> GPPPRFQRDFVDLRTDCPSTHPPIRVMQWNILAQALGEGKDNFVQCPVEALKWEERKCLILEEILAYQPDILCLQEVDHYFDTFQPLLSRLGYQGTFFPKPWSPCLDVEHNNGPDGCALFFLQNRFKLVNSANIRLTAMTLKTNQVAIAQTLECKESGRQFCIAVTHLKARTGWERFRSAQGCDLLQNLQNITQGAKIPLIVCGDFNAEPTEEVYKHFASSSLNLNSAYKLLSADGQSEPPYTTWKIRTSGECRHTLDYIWYSKHALNVRSALDLLTEEQIGPNRLPSFNYPSDHLSLVCDFSFTEESDGLS

A screen for circadian genes using Xenopus laevis retinas identified the ~50 kDa protein Nocturnin (NOCT), which exhibited a rhythmic expression that peaks at night (16 h Zeitgeber time, ZT16). NOCT is a member of the exonuclease/endonuclease/phosphatase family of proteins which include PDE12, a mitochondrial deadenylase needed for maturation of mitochondrial tRNAs, and CNOT6L, the mammalian ortholog of the main cytosolic yeast deadenylase CCR412,13. Thus, NOCT uses NADP+ and NADPH as substrates and removes the terminal 2′-phosphate. In conclusion, we propose that NOCT/Curled convert NADP+ to NAD+ and NADPH to NADH to regulate metabolism and in the case of NOCT, to synchronize metabolism with the biological clock.

To understand precisely how NOCT recognizes NADPH, we obtained co-crystals by using calcium instead of magnesium to inhibit the activity of WT NOCT and to stabilize the NOCT•NADPH complex. NOCT forms few contacts with the nucleobases. The adenine is sandwiched between two arginines (R290 and R367) via cation-pi interactions. The density for the adenine is relatively weak, indicating that these interactions are relatively dynamic. In contrast, the ribose-5′-PP-5′-ribose-2′-P backbone of NADPH forms multiple stable contacts and has better electron density. The 2′-P of NADPH is placed in a chemically ideal position for dephosphorylation. In NOCT, the phosphate coordinates with the catalytic metal ion, which is positioned to stabilize the leaving group (ribose oxygen). The orientation of the ribose near the catalytic metal ion places the 2′ ribose position rather than the 3′ ribose position for chemical attack. This can explain the inability of NOCT to cleave RNA. In the NOCT•NADPH complex, the α5β5 motif packs closely with the nicotinamide-bearing sugar.> TMSEIDRIAQNIIKSHLETCQYTMEELHQLAWQTHTYEEIKAYQSKSREALWQQCAIQITHAIQYVVEFAKRITGFMELCQNDQILLLKSGCLEVVLVRMCRAFNPLNNTVLFEGKYGGMQMFKAL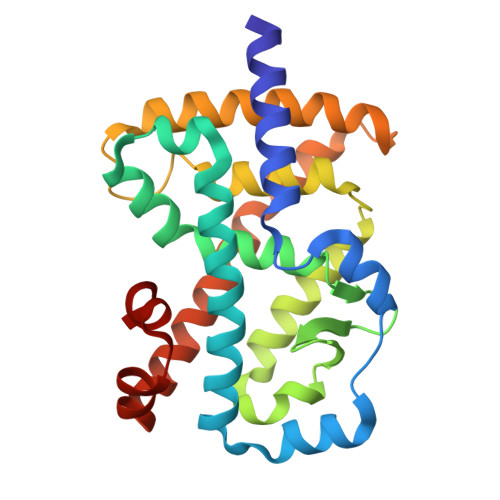GSDDLVNEAFDFAKNLCSLQLTEEEIALFSSAVLISPDRAWLLEPRKVQKLQEKIYFALQHVIQKNHLDDETLAKLIAKIPTITAVCNLHGEKLQVFKQSHPDIVNTLFPPLYKELFN> MTSNNLPTVLESIVEGRRGHLEEIRARIAHVDVDALPKSTRSLFDSLNQGRGGARFIMECKSASPSLGMIREHYQPGEIARVYSRYASGISVLCEPDRFGGDYDHLATVAATSHLPVLCKDFIIDPVQVHAARYFGADAILLMLSVLDDEEYAALAAEAARFDLDILTEVIDEEEVARAIKLGAKIFGVNHRNLHDLSIDLDRSRRLSKLIPADAVLVSESGVRDTET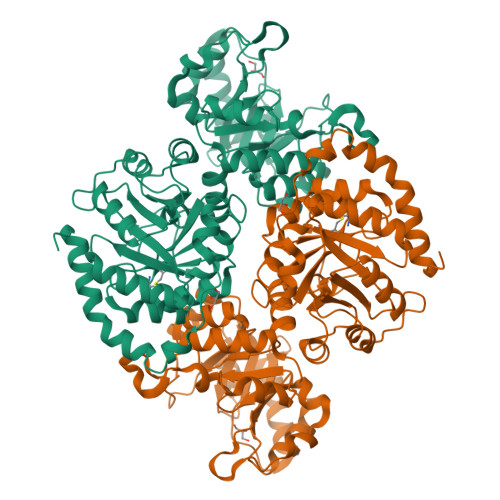VRQLGGHSNAFLVGSQLTSQENVDLAARELVYGPNKVCGLTSPSAAQTARAAGAVYGGLIFEEASPRNVSRETLQKIIAAEPNLRYVAVSRRTSGYKDLLVDGIFAVQIHAPLQDSVEAEKALIAAVREEVGPQVQVWRAISMSSPLGAEVAAAVEGDVDKLILDAHEGGSGEVFDWATVPAAVKAKSLLAGGISPDNAAQALAVGCAGLDINSGVEYPAGAGTWAGAKDAGALLKIFATISTFHYLEHHHHHH> MYSKVFLKPHCEPEQPAALPLFQPQLVQGGRPDGYWVEAFPFRSDSSKCPNIIGYGLGTYDMKSDIQMLVNPYATTNNQSSSWTPVPLAKLDFPVAMHYADITKNGFNDVIITDQYGSSMDDIWAYGGRVSWLENPGELRDNWTMRTIGHSPGMHRLKAGHFTRTDRVQVVAVPIVVASSDLTTPADVIIFTAPDDPRSEQLWQRDVVGTRHLVHEVAIVPAAETDGEMRFDQIILAGRDGVDCLWYDGARWQRHLVGTGLPEERGDPYWGAGSAAVGRVGDDYAGYICSAEAFHGNTVSVYTKPAGSPTGIVRAEWTRHVLDVFGPLNGKHTGSIHQVVCADIDGDGEDEFLVAMMGADPPDFQRTGVWCYKLVDRTNMKFSKTKVSSVSAGRIATANFHSQGSEVDIATISYSVPGYFESPNPSINVFLSTGILAERLDEEVMLRVVRAGSTRFKTEMEFLDVAGKKLTLVVLPPFARLDVERNVSGVKVMAGTVCWADENGKHERVPATRPFGCESMIVSADYLESGEEGAILVLYKPSSTSGRPPFRSMDELVAHNLFPAYVPDSVRAMKFPWVRCADRPWAHGRFKDLDFFNLIGFHVNFADDSAAVLAHVQLWTAGIGVSAGFHNHVEASFCEIHACIANGTGRGGMRWATVPDANFNPDSPNLEDTELIVVPDMHEHGPLWRTRPDGHPLLRMNDTIDYPWHAWLAGAGNPSPQAFDVWVAFEFPGFETFSTPPPPRVLEPGRYAIRFGDPHQTASLALQKNDATDGTPVLALLDLDGGPSPQAWNISHVPGTDMYEIAHAKTG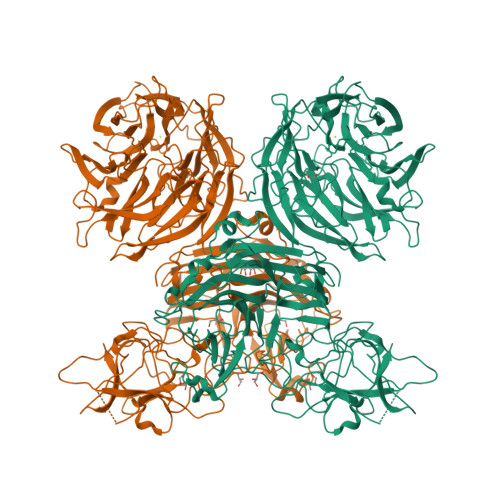SLVCARWPPVKNQRVAGTHSPAAMGLTSRWAVTKNTKGQITFRLPEAPDHGPLFLSVSAIRHQQEADAIPVIVQGDSIELSAWSLVPAN> MAHHHHHHMNCNYNCVTLHNSVRMPQLGLGVWRAQDGAETANAVRWAIEAGYRH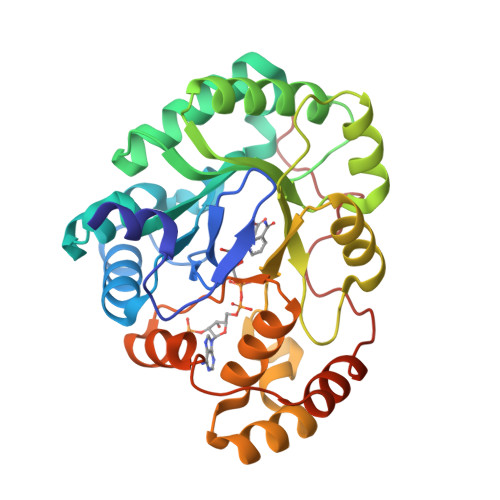IDTAYIYSNERGVGQGIRESGVPREEVWVTTKVWNSDQGYEKTLAAFERSRELLGLEYIDLYLIHWPGKKKFVDTWKALEKLYEEKKVRAIGVSNFEPHHLTELFKSCKIRPMVNQVELHPLFQQRTLREFCKQHNIAITAWSPLGSGEEAGILKNHVLGEIAKKHNKSPAQVVIRWDIQHGIVTIPKSTNKGRIQENFNVWDFKLTEEEMRQIDELNEDKRIGADPDNFFPGGEE> 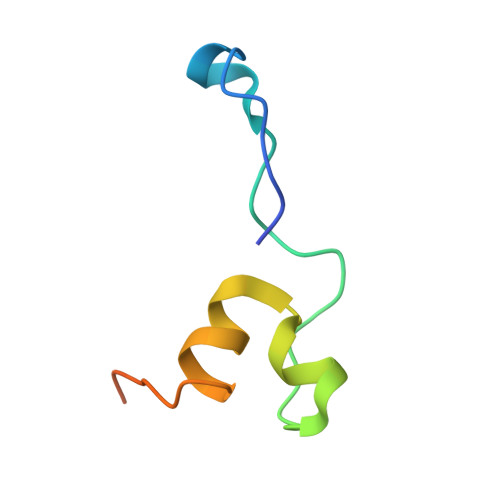XMEPVDPRLEPWKHPGSQPKTACTNCYCKKCCFHCQVCFITKALGISYGRKKRRQRRR> GAHMDCHLSDMLQQLHSVNASKPSERGLVRQEEAEDPACIPIFWVSKWVDYSDKYGLGYQLCDNSVGVLFNDSTRLILYNDGDSLQYIERDGTESYLTVSSHPNSLMKKITLLKYFRNYMSEHLLKAGANITPREGDELARLPYLRTWFRTRSAIILHLSNGSVQINFFQDHTKLILCPLMAAVTYIDEKRDFRTYRLSLLEEYGCCKELASRLRYARTMVDKLLSSRSASNRLKA;> LHSTA

The human polo-like kinase 1 (PLK1) is a key regulator of chromosome segregation during mitosis, through its essential biological functions in chromosome condensation, cohesin dissociation from chromosomes, mitotic entry, centrosome maturation, kinetochore function, spindle assembly, and exit from mitosis. The PBD recognizes phospho (p)Ser/Thr protein substrates for the kinase catalytic activity of PLKs12. Intriguingly, recent crystallographic studies have identified a hydrophobic pocket within the human PLK1 PBD, located adjacent to the phosphosubstrate binding groove, which may regulate substrate recognition. Seven hydrophobic amino acid residues line the pocket; whilst V415, L478, and F482 cover the bottom of the pocket, the Tyr residues Y417, Y421, Y481 and Y485, form its sides.

The pocket is evident only in certain structural conformers, suggesting that it may adopt an open conformation in which it could accommodate residues from PLK1 substrates, or alternatively, a closed conformation precluding such interactions. The proximity of the Tyr pocket to the phosphosubstrate binding groove, and its ability to adopt an open conformation, suggest that it may assist in the recognition of PBD substrates that contain hydrophobic side chains, enabling substrate discrimination.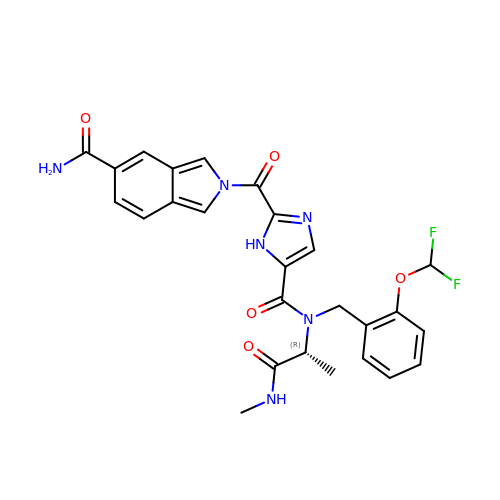2-[[5-[[2-[bis(fluoranyl)methoxy]phenyl]methyl-[(2~{R})-1-(methylamino)-1-oxidanylidene-propan-2-yl]carbamoyl]-1~{H}-imidazol-2-yl]carbonyl]isoindole-5-carboxamide | C26 H24 F2 N6 O5 | QTSQRRSNHSLXPH-CQSZACIVSA-N>ACVNQCPDAIDRFIVKDKGCHGVEKKYYKQVYVACMNGQHLY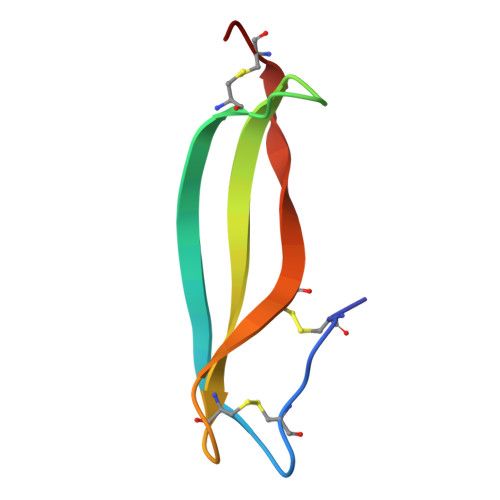CRTEWGGPCQL[2x]>MANANQVALGRSNLSTGTGYGGATDKYALYLKLFSGEMFKGFQHETIARDLVT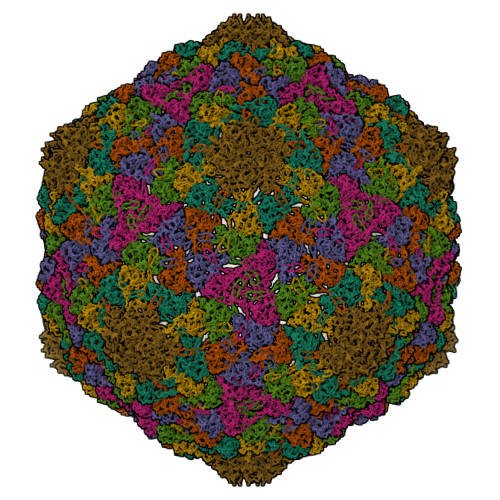KRTLKNGKSLQFIYTGRMTSSFHTPGTPILGNADKAPPVAEKTIVMDDLLISSAFVYDLDETLAHYELRGEISKKIGYALAEKYDRLIFRSITRGARSASPVSATNFVEPGGTQIRVGSGTNESDAFTASALVNAFYDAAAAMDEKGVSSQGRCAVLNPRQYYALIQDIGSNGLVNRDVQGSALQSGNGVIEIAGIHIYKSMNIPFLGKYGVKYGGTTGETSPGNLGSHIGPTPENANATGGVNNDYGTNAELGAKSCGLIFQKEAAGVVEAIGPQVQVTNGDVSVIYQGDVILGRMAMGADYLNPAAAVELYIGATAPSAF[7x]>MAAVLESLLREEVSVAAVVRWIARSTQGSEDNAGEAAALSSLRALRKEFVPFLLNFLREQSSRVLPQGPPTPAKTPGASAALPGRPGGPPRGSRGARSQLFPPTEAQSTAAEAPLARRGGRRRGPGPARERGGRGLEEGVSGESLPGAGGRRLRGSGSPSRPSLTLSDPPNLSNLEEFPPVGSVPPGPTGTKPSRRINPTPVSEERSLSKPKTCFTSPPISCVPSSQPSALDTSPWGLGLPPGCRSLQEEREMLRKERSKQLQQSPTPTCPTPELGSPLPSRTGSLTDEPADPARVSSRQRLELVALVYSSCIAENLVPNLFLELFFVFQLLTARRMVTAKDSDPELSPAVLDSLESPLFQSIHDCVFFAVQVLECHFQVLSNLDKGTLKLLAENERLLCFSPALQGRLRAAYEGSVAKVFLVMPPSTQAVSFQPETDNRANFSSDRAFHTFKKQRDVFYEVLREWEDHHEEPGWDFEKGLGSRIRAMMGQLSAACSHSHFVRLFQKQLLQMCQSPGGAGGTVLGEAPDVLSMLGADKLGRLWRLQERLMAPQSSGGPCPPPTFPGCQGFFRDFILSASSFQFNQHLMDSLSLKIQELNGLALPQHEPNDEDGESDVDWQGERKQFAVVLLSLRLLAKFLGFVAFLPYRGPEPPPTGELQDSILALRSQVPPVLDVRTLLQRGLQARRAVLTVPWLVEFLSFADHVVPLLEYYRDIFTLLLRLHRSLVLSQESEGKMCFLNKLLLLAVLGWLFQIPTVPEDLFFLEEGPSYAFEVDTVAPEHGLDNAPVVDQQLLYTCCPYIGELRKLLASWVSGSSGRSGGFMRKITPTTTTSLGAQPSQTSQGLQAQLAQAFFHNQPPSLRRTVEFVAERIGSNCVKHIKATLVADLVRQAESLLQEQLVTQGEEGGDPAQLLEILCSQLCPHGAQALALGREFCQRKSPGAVRALLPEETPAAVLSSAENIAVGLATEKACAWLSANITALIRREVKAAVSRTLRAQGPEPAARGERRGCSRACEHHAPLPSHLISEIKDVLSLAVGPRDPDEGVSPEHLEQLLGQLGQTLRCRQFLCPPAEQHLAKCSVELASLLVADQIPILGPPAQYRLERGQARRLLHMLLSLWKEDFQGPVPLQLLLSPRNVGLLADTRPREWDLLLFLLRELVEKGLMGRMEIEACLGSLHQAQWPGDFAEELATLSNLFLAEPHLPEPQLRACELVQPNRGTVLAQSLEACGTKLENLYFQ[2x];>[3x]GSMAKVQVNNVVVLDNPSPFYNPFQFEITFECIEDL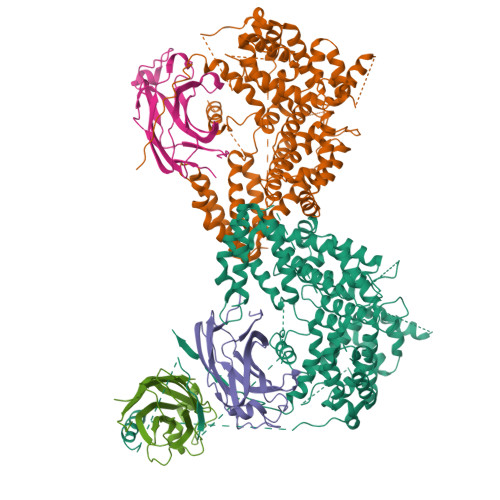SEDLEWKIIYVGSAESEEYDQVLDSVLVGPVPAGRHMFVFQADAPNPGLIPDADAVGVTVVLITCTYRGQEFIRVGYYVNNEYTETELRENPPVKPDFSKLQRNILASNPRVTRFHINWEDNTEKLEDAESSNPNLQS> GSHMASMSKDEVKREAKDTDGN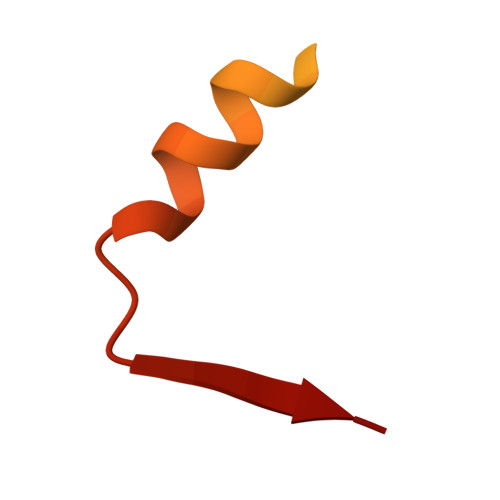PEIKGERRRLHSEIQSGSLANNIKKSTVIVKN>MISAKTLRPAIAAIALFAIGATGAWAQDKITVTSEKPVAAADVPADAVVVGIEKMKYLTPEVTIKAGETVYWVNGEVMPHNVAFKKGIVGEDAFRGEMMTKDQAYAITFNEAGSYDYFCTPHPFMRGKVIVE[2x];>[2x]MASARESTPRYLTLIGATLACSALALGAAQAQTEPAEPEAPAETAAADAAGQTEGQRGAAEAAAALAAGEADEPVILEAPAPDARRVYIQDPAHFAAITQQFVIDGSTGRILGMTDGGFLPHPVAAEDGSFFAQASTVFERIARGKRTDYVEVFDPVTFLPIADIELPDAPRFLVGTYQWMNALTPDNKNLLFYQFSPAPAVGVVDLEGKTFDRMLDVPDCYHIFPASPTVFYMNCRDGSLARVDFADGETKVTNTEVFHTEDELLINHPAFSLRSGRLVWPTYTGKIFQADLTAEGATFRAPIEALTEAERADDWRPGGWQQTAYHRQSDRIYLLVDQRDEWKHKAASRFVVVLNAETGERINKIELGHEIDSINVSQDAEPLLYALSAGTQTLHIYDAATGEELRSVD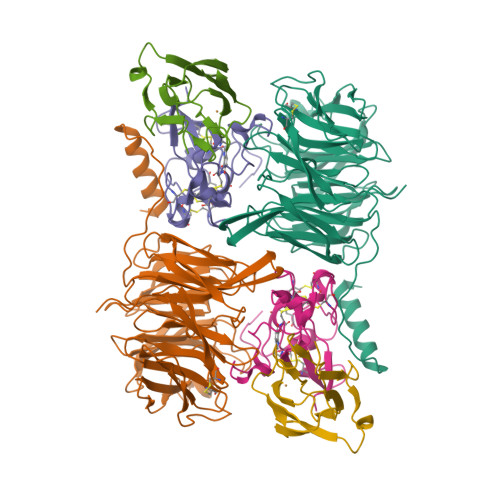QLGRGPQIITTHDMDS;>MLGNFRFDDMVEKLSRRVAGRTSRRGAIGRLGTVLAGAALVPLLPVDRRGRVSRANAAGPAEGVDPRAKWQPQDNDIQACDYWRHCSIDGNICDCSGGSLTNCPPGTKLATASWVASCYNPTDGQSYLIAYRDCCGYNVSGRCPCLNTEGELPVYRPEFANDIIWCFGAEDDAMTYHCTISPIVGKAS[2x]> VTA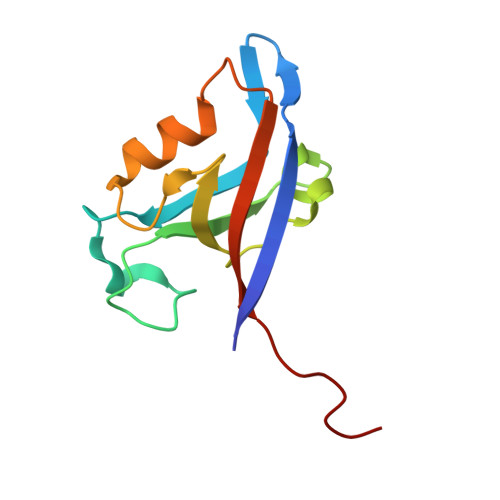VVQRVEIHKLRQGENLILGFSIGGGIDQDPSQNPFSEDKTDKGIYVTRVSEGGPAEIAGLQIGDKIMQVNGWDMTMVTHDQARKRLTKRSEEVVRLLVTRQSLQKAVQQ> MSQQENPKYLWWNHRIIPWEEATVHLTDYWWASVTAVFEVISGYWNNAEGEMYIFRLEDHARRLEQSMQLIRMPKEFTVDEICQATIDLVRANDYRGDVFIMPLAYAVGNKAFRVVGDRTTEMFIYSRPAVSRLEEDFSLHACYSSWTRINERVLPPRIKALANYRNSQLASSEAAMNGYDTALFLNPEGKVAEGTGSCVFFVRKGKLITPDITSGILESITRDTVIHLAREVLGLEVEERVVDRTETYLADEAFLCGTHAEITPIASIDRHEMKHGAPGPITRQLRDIYREVVYGRDFRYRNWLTPVGMGVRAEQ

Transaminases (TAs; aminotransferases; EC 2.6.1.) are pyridoxal-5’-phosphate (PLP)-dependent enzymes that catalyze the reversible stereoselective transfer of an amino group from an amino substrate to a keto acid or ketone, thereby producing a chiral amine or amino acid and a new keto compound. TaTT is distinguished by an expanded substrate specificity: it can catalyze the amino group transfer between BCAAs and α-ketoglutarate, producing α-keto acids and L-glutamate (benchmark reactions for BCATs), and between R-PEA and α-ketoglutarate producing ketone and L-glutamate (R-TA-like activity). The functional dimer of TaTT is close to the dimers of known BCATs; however, the P-pocket comprises only one site for the α-COOH group binding, and the O-pocket is enriched with hydrophobic residues, which disturb the alternation of hydrophobic and hydrophilic residues typical of BCATs. Generally, the active site is a combination of two pockets: the O-pocket on the phenolic side of the PLP and the P-pocket on the phosphate group side of the PLP.

The mP3O1 variant, harboring a triple mutation in the P-pocket and the mutation S115R in the O-pocket loop, showed the highest affinity to R-PEA. The variant mP3O1 showed the highest specificity for R-PEA: three mutations in the P-pocket together with a mutation S115R in the O-pocket loop improved the productive binding of R-PEA as well as the effectiveness of the amino group transfer. It is noteworthy that the achieved effect was not a sum of the effects induced by the separate mutations in the P-pocket (mP1 + mP2) and O-pocket (mO1); rather, it was the cumulative effect of the four mutations (G41V + Y101F + R43S + S115R). Mutation R43S in both variants led to a shift of the β-turn and the interdomain loop toward the active site: about 0.6 Å between the corresponding Cα atoms of H261 and V132. Substitution of a side chain of R43 induced the flexibility of the H261 side chain in both variants, which is reflected by the high B-factor (mP3) or even the absence of the electron density for the side chain (mP3O1). There are large conformation changes in the O-pocket loop in the mP3 and mP3O1 variants; moreover, in mP3O1, this loop is partially disordered (residues 113–117 have no clear electron density). The S115R mutation in the O-pocket loop induced its disordering and increased the W32* side chain flexibility. In mP3O1 (mP3 + S115R), W32* has two conformations: one is similar to that in mP3, and the other is unique and occupies the WT position of the O-pocket loop main chain. As an imitation of the R-TAs’ pyruvate-binding site, the introduction of S115R in mP3 was unsuccessful: the productive binding of pyruvate in the proD-position (through the coordination of the α-COOH group with the side chain of R115 in the O-pocket loop) was not achieved. The HPLC analysis of the products of transamination between R-PEA and pyruvate catalyzed by mP3O1 revealed only L-alanine.> MNLEAKKKVLRSFTYGLYVLTAKDGDEV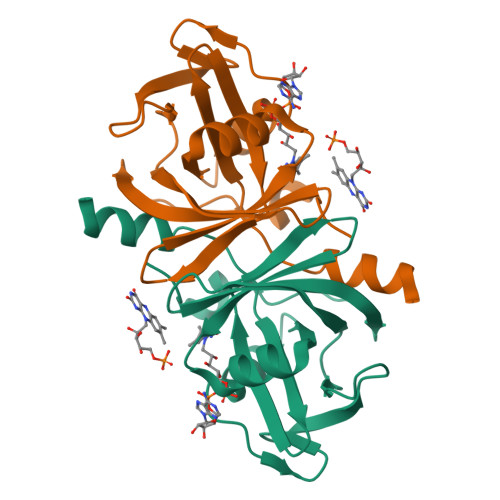AAGTVNWVTQASFQPPLVAVGLKRDSHLHALVERTGKLALMTLAHDQKAIAQDFFKPTVREGDRLNGHPFEPSPTFGLPLLTELPYWLEAEVRHLYPGGDHSLVVAEVVEAGVRREEKPLVMWDTGWFYGG> GTA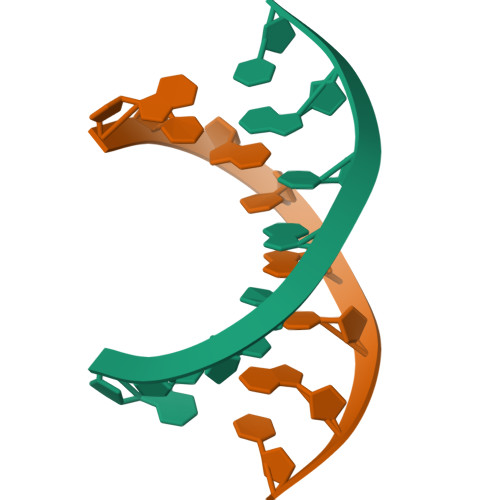CGTAC> MRGSHHHHHHGSVEYTPWLIAGLGNP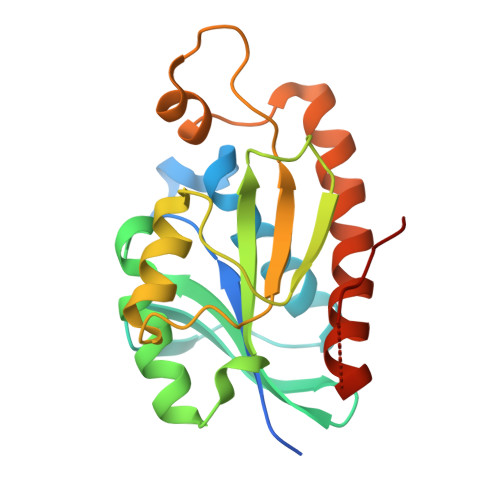GNKYYGTRHNVGFEMVDRIAAEEGITMNTIQSKSLLGIGSIGEVPVLVVKPQSYMNYSGEAIGPLAAYYQVPLRHILLIYDDTSLPNGVLRLQKKGGHGRHNGLQNVIEHLDGRREFPRLSIGIGSPPGKMDPRAFLLQKFSSEERVQIDTALEQGVDAVRTLVLKGFSGSTERFNLVQ Here we report the neutron crystal structure of a PLP-dependent enzyme, aspartate aminotransferase (AAT), a fold-type I PLP-dependent enzyme that reversibly converts l-aspartate and α-ketoglutarate to oxaloacetate and l-glutamate via a ping−pong bi−bi mechanism. Pyridoxal 5′-phosphate (PLP), the biologically active cofactor derived from pyridoxine, is one of the most ubiquitous cofactors found in nature, catalyzing ~140 different types of biochemical transformations. Recombinant porcine cytosolic AAT fortuitously packs as a biological and crystallographic homodimer, with the two active sites having different activities toward the substrate analog α-methylaspartic acid. In AAT, the protonated pyridine nitrogen of the PLP (N1-PLP) enhances charge delocalization through resonance, permitting the subsequent transamination reaction.

Thus, in the room-temperature neutron structure of AAT, after the crystal was soaked with α-methylaspartic acid, one site reacts and closes (chain A), whereas the second one remains unreacted and open (chain B). In the open monomer, the Schiff base (SB) is in the internal aldimine form and PLP is covalently linked to a conserved lysine residue (K258). The closed monomer displays the SB in the external aldimine form, with PLP covalently linked to the Cα of α-methylaspartate. The out-of-plane geometry for the SB observed in our neutron structure was also identified in other aminotransferase enzymes, with torsion angles ranging from 43 to 96°13. Overall, the experimental evidence demonstrates that O3′ and the SB are deprotonated and likely carry partial negative charges, stabilized by PLP resonance and H bonds with Y225 and N194. More importantly, the SB C=N double bond is 46° above the plane of the pyridinium ring, which indicates the lack of a hydrogen bond to O3′. A strong nuclear scattering length density peak for a deuterium appears near the NSB in the external aldimine (chain A), indicating that the SB is protonated. Remarkably, the peak is not between O3′ and NSB, but is instead located between NSB and the C-terminal carboxylate oxygen of α-methylaspartate. We found a deuteron positioned equidistant between the NSB nitrogen and oxygen of the substrate C terminus oxygen in the external aldimine, indicative of a low-barrier hydrogen bond (LBHB). The neutron structure shows that K258 is neutral (ND2), corroborating its role as the general base catalyst. Moreover, in the internal aldimine, H143 and H189 are neutral, while in the external aldimine H143 remains neutral but H189 becomes protonated and positively charged.

>[2x]APPSVFAEVPQAQPVLVFKLIADFREDPDPRKVNLGVGAYRTDDCQPWVLPVVRKVEQRIANNSSLNHEYLPILGLAEFRTCASRLALGDDSPALQEKRVGGVQSLGGTGALRIGAEFLARWYNGTNNKDTPVYVSSPTWENHNGVFTTAGFKDIRSYRYWDTEKRGLDLQGFLSDLENAPEFSIFVLHACAHNPTGTDPTPEQWKQIASVMKRRFLFPFFDSAYQGFASGNLEKDAWAIRYFVSEGFELFCAQSFSKNFGLYNERVGNLTVVAKEPDSILRVLSQMQKIVRVTWSNPPAQGARIVARTLSDPELFHEWTGNVKTMADRILSMRSELRARLEALKTPGTWNHITDQIGMFSFTGLNPKQVEYLINQKHIYLLPSGRINMCGLTTKNLDYVATSIHEAVTKIQ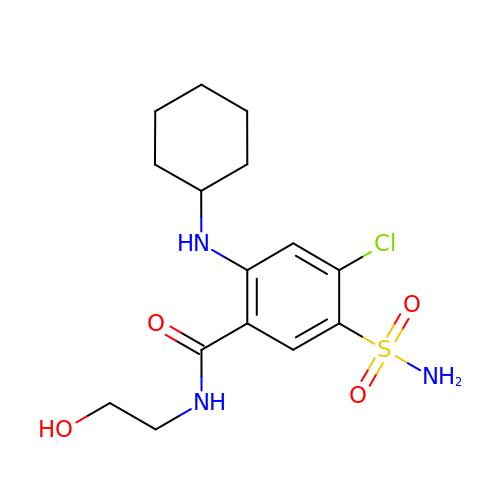4-chloranyl-2-(cyclohexylamino)-~{N}-(2-hydroxyethyl)-5-sulfamoyl-benzamide | C15 H22 Cl N3 O4 S | MDLHQNNKYAWRKZ-UHFFFAOYSA-N> ASHQNINQFKREVAKIDTNTVERRIALANAYNETLSRNPLLIDPFTSKQKEGLREYARMLEVHEQIGHVAIPSIGVDI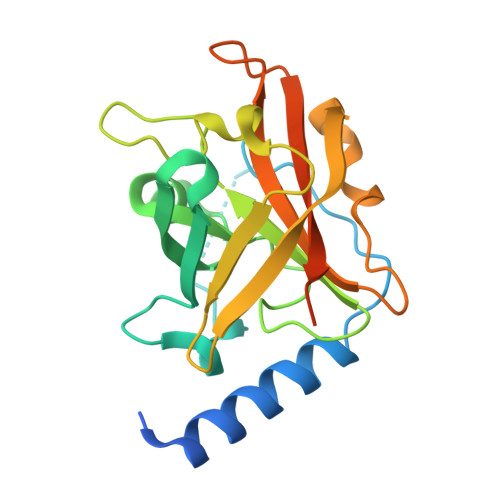PIYAGTSETVLQKGSGHLEGTSLPVGGLSTHSVLTAHRGLPTARLFTDLNKVKKGQIFYVTNIKETLAYKVVSIKVVDPTALSEVKIVNGKDYITLLTCTPYMINSHRLLVKGERIPYDSTEAEKHKEQTVQDYRLS> GAHMNIQKIQIKFQPIGSIGQLKPSVCKISMSQSFAMVILFLKRRLKM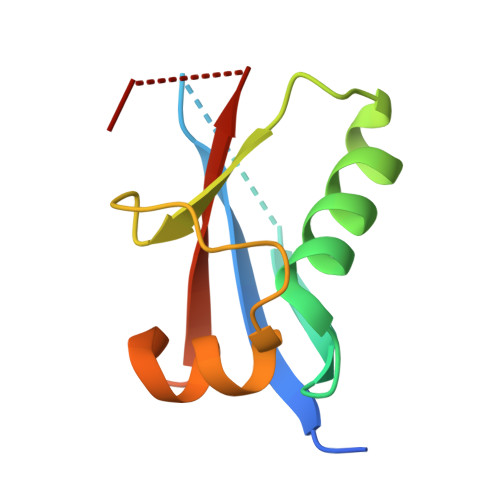DHVYCYINNSFAPSPQQNIGELWMQFKTNDELIVSYCASVAFG> GPLMDNETQIKKRKLQTATMEAKATGEIFVVPFFGQGHLFPAMELCKNISAHNYNVTLIIPSHLSSSIPSTFSNHSSFIHVTEISVAASPPPEAADEPGSGTEVRSSGPRGNPLQDQNLQMGKGIKSFLSARSGTRPTCVVIDVMMSWSKEIFVDHEIPVVSFSTSGATASAVGYGMWKAEVGNMKPGEIREIPGLPKEMAVTFADLSRGPQRRIRPPGGPGKSDGRAGPPNRMRSGSRHGPGGGPSPGPGQKPRWVDEVDGSIALLINTCDDLEHVFINYMAEQTKLPVWGVGPLLPEQFWKSAGELLHDHEMRSNHKSNYTEDEVVQWLESKPRESVIYISFGSE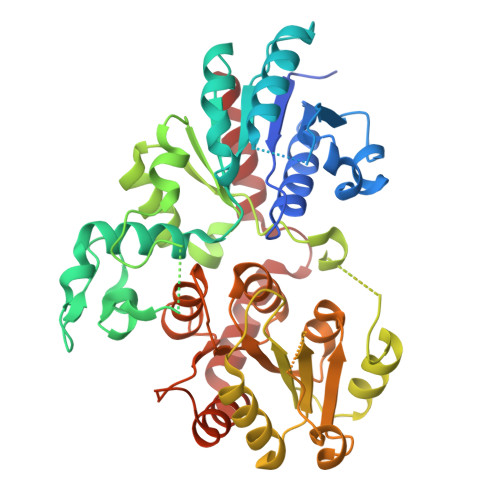VGPTIEEYKELAKALEESDQPFIWVIQPGSGKSGIPRSFLGPAAAHTDDSEEEEGYYPDGLDVTVGNRGLIITGWAPQLLILSHPSTGGFLSHCGWNSTAEAIGRGVPILGWPIRGDQFDNAKLVAYHLKIGHVMSRGANGEVGPGKFTKDDITSGIEKLMKDEKVHKQAKELSKEFEGGFPVSSVKALGAFVEFISQKAT> GQAFRKFLPLFDRVLVERSAAETVTKGG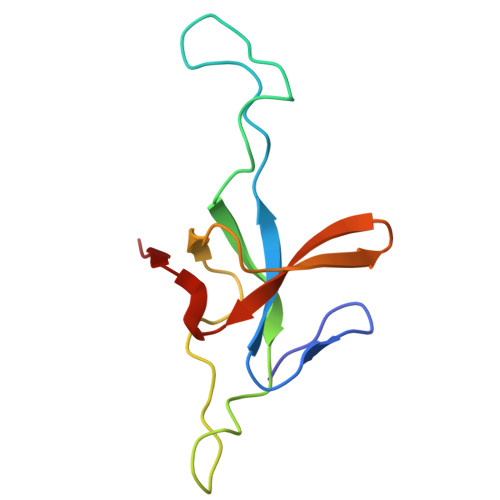IMLPEKSQGKVLQATVVAVGSGSKGKGGEIQPVSVKVGDKVLLPEYGGTKVVLDDKDYFLFRDGDILGKYVD> GSAQVPQGHCEEHLDPLSIYCEQDRTLVCGVCASLGSHRGHRLLPAAEAQARLKTQLPQQKMQLQEASMRKEKTVAVLEHQLVEVEETVRQFRGAVGEQLGKMRMFLAALESSLDREAERVRGDAGVALRRELSSLNSYLEQLRQMEKVLEEVADKPQTEFLMKFSLVTSRLQKILSESPPPARLDIQLPVISDDFKFQVWKHMFRHLMPALEELTFDPSSAHPSLVVSSSGRRVECSDQKAPPAGEDTRQFDKAVAVVAQQLLSQGEHYWEVEVGDKPRWALGVMAADASRRGRLHAVPSQGLWLLGLRDGKILEAHVEAKEPRALRTPERPPARIGLYLSFADGVLAFYDASNPDVLTPIFSFHERLPGPVYPIFDVCWHDKGKNAQPLLLV

Tripartite motif-containing protein (TRIM)72 (mitsugumin 53; MG53) has been determined to rapidly nucleate vesicles at the site of membrane damage, but the underlying molecular mechanisms remain poorly understood. Here we present the structure of Mus musculus TRIM72, a complete model of a TRIM E3 ubiquitin ligase. TRIM72 is a member of the class IV TRIM proteins, which is the largest subtype among the 11 groups of TRIM proteins. Its domain organization includes an RBCC domain followed by a PRY motif associated with a SPRY domain identified in splA kinase and ryanodine receptors (PRYSPRY) domain.

After introducing point mutations and deletions, we were finally able to resolve molecular models of mouse TRIM72, including RING-deleted (ΔRING, 2.75 Å; the highest resolution is in parentheses), full-length (FL, 4.6 Å) and wild-type (WT, 7.1 Å) TRIM72. The overall structure of the TRIM72 dimer has an elongated shape. The coiled-coil domains (CCDs) form the main scaffold of an antiparallel dimer with a length of approximately 17 nm. In the middle of the CCDs, the structural core consists of the hendecad repeated region of the H1:H1′ helices (prime indicates the second protomer of the dimer) and the H3:H3′ helices followed by a pair of PRYSPRY domains. One side of the H3:H3′ helices is wrapped in a four-helical bundle with the hendecad H1:H1′ helices, and the other side contacts the β-sheet of PRYSPRY through hydrophobic interfaces, hydrogen bonding and ionic interactions. PRYSPRY comprises two antiparallel β-sheets: one sheet (β3, β5–β8 and β12) forms a concave surface, and the other sheet (β1, β2, β4, β9–β11 and β13) forms a convex surface. First, several arginines (R356, R368, R369, R371 and R386) and lysines (K317, K330, K389, K398, K460 and K462) are situated on the concave surface, consisting of variable loops (VLs), and contribute to its positive charge. Second, each PRYSPRY domain displays a concave surface that is positively charged toward the same side, facing opposite the CCDs. Recent cryo-electron microscopy (EM) analysis of TRIM72 and the crystal structure of TRIM72 ΔRING also revealed that the CCD ends are dynamic.> SLSNKLTL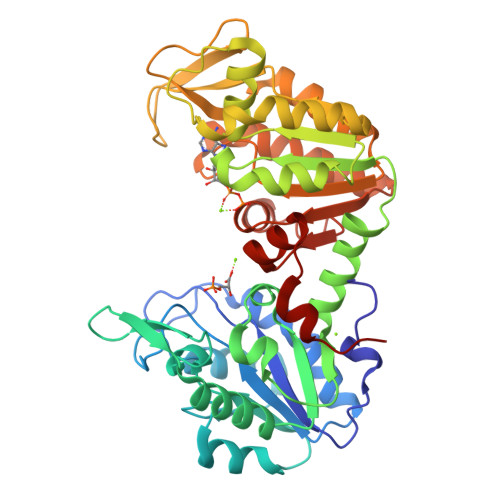DKLDVKGKRVVMRVDFNVPMKNNQITNNQRIKAAVPSIKFCLDNGAKSVVLMSHLGRPDGVPMPDKYSLEPVAVELKSLLGKDVLFLKDCVGPEVEKACANPAAGSVILLENLRFHVEEEGKGKDASGNKVKAEPAKIEAFRASLSKLGDVYVNDAFGTAHRAHSSMVGVNLPQKAGGFLMKKELNYFAKALESPERPFLAILGGAKFADKIQLINNMLDKVNEMIIGGGMAFTFLKVLNNMEIGTSLFDEEGAKIVKDLMSKAEKNGVKITLPVDFVTADKFDENAKTGQATVASGIPAGWMGLDCGPESSKKYAEAVTRAKQIVWNGPVGVFEWEAFARGTKALMDEVVKATSRGCITIIGGGDTATCCAKWNTEDKVSHVSTGGGASLELLEGKVLPGVDALSNI Smad proteins consist of an N-terminal MH1 domain, which binds to DNA, a linker region with phosphorylation sites for network regulatory inputs, and a C-terminal MH2 domain that is phosphorylated by the receptors and binds other Smad proteins, LDTFs, chromatin readers, and transcriptional co-activators and co-repressors. The receptors for TGF-β, nodal, activin, myostatin, and other family members are membrane serine/threonine kinases that phosphorylate and activate Smad2 and Smad3, whereas analogous receptors for the bone morphogenetic proteins (BMPs) preferentially phosphorylate and activate Smads 1, 5, and 8. These receptor-activated Smads (R-Smads) form heterotrimeric complexes with Smad4, which is required for the transcriptional regulation of most target genes. Focusing on the human and mouse Gsc promoter, here we identify specific Smad-binding GC-rich motifs and provide the X-ray crystal structures of Smad3 and Smad4 bound to several of these motifs. The structures determined here reveal that the β-hairpin is flexible and adaptable to bind with high-affinity several variants of the consensus sequence GGC(GC)|(CG), which we refer to as 5GC SBE.

Next, we investigated the binding mode of the Smad3 MH1 domain with the GGCGC motif. Crystals of human Smad3 MH1 domain bound to a 16mer dsDNA oligonucleotide containing the GGCGCG motif yielded data at 2.05 Å resolution using synchrotron radiation (I41 symmetry ID29, ESRF, Grenoble), which together with the Smad4 bound to the same site, are the highest-resolution structures determined for a DNA-bound Smad MH1 domain to date. The asymmetric unit (ASU) of the complex contains two Smad3 monomers and one dsDNA. As in all other MH1 complexes, the three residues strictly conserved (Arg74 and Gln76 located in β2 and Lys81 in β3) are well defined in the structure and participate in a network of hydrogen bonds with the 5-GGCGCG-10 motif. The guanidine group of Arg74 is well ordered due to its tight coordination by the G5 nucleotide (fitting of the side chains to the density are shown in Fig. 4i). The Lys81 side chain is also well defined, through hydrogen bond interactions from the ɛ-amino group to the pair of nucleotides G6 and G10′ (in the complementary chain) and with several well-ordered water molecules in the proximity of the ɛ-amino group. The Gln76 side chain carbonyl interacts with N3 of C9′, and also with C7, G8, and G8′ mediated by the presence of several tightly bound water molecules. Various interactions occurred between Leu71, Gln76, Ser78, His79, and His101 backbone and the DNA phosphates. In fact, Smad3 and Smad4 GGCGC complexes are structurally very similar with a Cα RMSD of 0.44 Å for 105 aligned residues and both complexes interact directly with the DNA using the β2–β3 hairpin.

>GAMIVKRLLGWKKGEQNGQEEKWCEKAVKSLVKKLKKTGQLDELEKAITTQNVNTKCITIPRSLDGRLQVSHRKGLPHVIYCRLWRWPDLHSHHELRAMELCEFAFNMKKDEVCVNPYHYQRVETPVL[2x]> GPGMLSILLSASSSYQTQTIGRLTTPGTNLVKAYKSSNPDLARNCYWLYFDY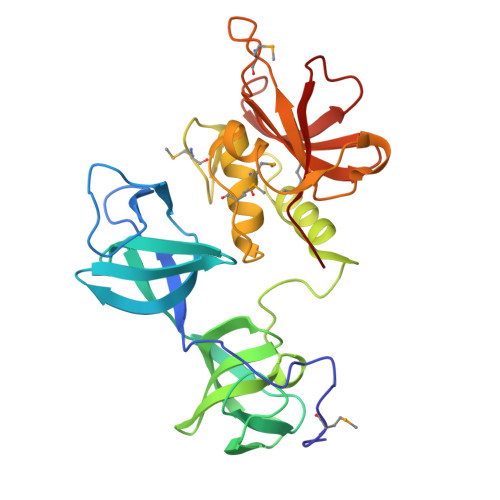YVHILGYENGFAHVRIGTEDCWISKDSLEEITIPTQSVTEANIYSEPSRTGTIVRYVPANSQVTILDFNCDGFYRINYRGYIGYILEDALQYKWKQIDGANDGERAANLVKTKLGCKYILGMSGPDTYDCSGLMQWAYNRLDIFMHRTADVQDLHGQLIEDAQDILPGDIITFRTDSDNPMLVTHVGMYVGNGQFIHASTNGYVVKYQDFYKYPYPVSTIRRYWTK>[5x]GGVEVLEVKTGVDAITEVECFLNPEMGDPDENLRGFSLKLSAQNDFSSDSPERKMLPCYSTARIPLPNLNEDLTSGNLLMWEAVTVQTEVIGITSMLNLHAGSQKVHEHGGGKPIQGSNFHFFAVGGEPLEMQGVLMNYRSKYPDGTITPKNPTAQSQVMNTDHKAYLDKNNAYPVECWVPDPSRNENARYFGTFTGGENVPPVLHVTNTATTVLLDEQGVGPLCKADSLYVSAADICGLFTNSSGTQQWRGLARYFKIRLRKRSVKNPYP

BK polyomavirus (BKPyV) is a small, non-enveloped, double-stranded DNA virus with an icosahedral capsid formed by 72 capsomers, where a capsomer is an association of a pentamer of the VP1 protein linked internally to a single copy of either the VP2 or the VP3 proteins. BK polyomavirus (BKPyV) is an opportunistic pathogen that uses the b-series gangliosides GD1b and GT1b as entry receptors. Viruses sampled sequentially from these patients accumulated multiple mutations in the BC loop region of the VP1 protein, which is involved in the direct interaction of the virus with sialic acids. All variant VP1 pentamer structures were globally similar to the WT VP1 pentamer with a doughnut-shaped ring composed of a central pore surrounded by five VP1 monomers in 5-fold symmetry.

The E73Q pentamer structure was almost identical to that of the WT (RMSD in the BC loop region, from amino acids 68–76, of 0.5 Å), whereas the E73A mutant presenting an alanine in the same position showed some structural changes. Mutation of the initial glutamic acid at position 73 to glutamine in the E73Q variant did not modify the orientation of the BC loop, while its mutation to alanine, in E73A, revealed the flexibility of this part of the BC loop. In addition to GD1b and GT1b, they showed binding to the ganglio-NGL probes that contain α2-3-linked sialic acid at the non-reducing end galactose as in GM1b-DH and GD1a-DH. The two variants having E to Q mutation at position 73, E73Q and VQQ bound, moreover, to a wider range of gangliosides of both a- and b-series including GD1a, GT1a, GD3, and GQ1b. The overall binding intensities for E73Q and VQQ VP1s were higher compared with the E73A and the WT VP1s. As expected, infection was seen for WT in cells supplemented with GD1b, but also for E73Q and E73A PSVs under the same condition, and infection was also seen for E73Q when cells were supplemented with GD1a in both LNCaP and GM95 cells. The ability of the E73Q variant to infect cells supplemented with GD1a was consistent with its increased infectivity in RS cells, which carried GD1a gangliosides. On the other hand, only variant E73Q showed strongly enhanced infectivity in RS cells, which as shown by mass spectroscopy, carried the GD1a ganglioside, and only variant E73Q was able to infect LNCaP and GM95 cells supplemented with GD1a. Similarly, in 293TT cells, E73Q retained infectivity equivalent to that of WT VP1, whereas both VQQ and E73A showed significantly reduced infectivity. Therefore, flipping of the BC2 loop, and not loss of negative charge at position 73, was correlated with loss of infectivity in 293TT cells. This led us to a model in which the two different structural effects of VP1 mutations at position 73 have opposite effects on infectivity: loss of charge increases infectivity, by broadening ganglioside binding, whereas BC loop flipping reduces infectivity.> IPEYVDWRQKGAVTPVKNQGSCGSCWAFSAVVTIEGIIKIRTGNLNQYSEQELLDCDRRSYGCNGGYPWSALQLVAQYGIHYRNTYPYEGVQRYCRSREKGPYAAKTDGVRQVQPYNQGALLYSIANQPVSVVLQAAGKDFQLYRGGIFVGPCGNKVDHAVAAVGYGPNYILIKNSWGTGWGENGYIRIKRGTGNSYGVCGLYTSSFYPVKN;>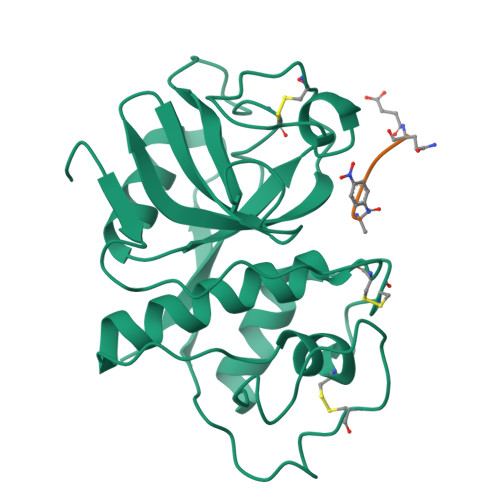 QVVAAX> GC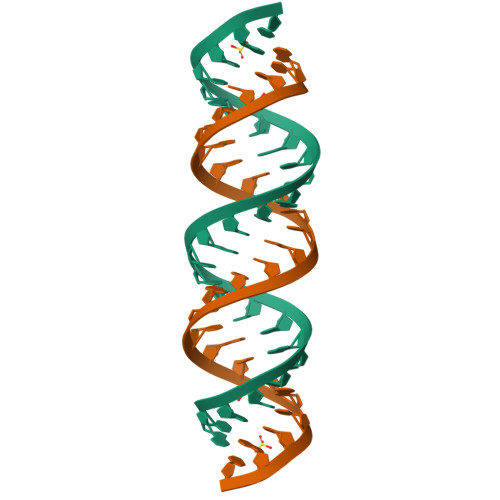UGCUGCUGCUGCUGCUGCUGCUGC>[2x]MAYFDYTSAKPVDERILEAMLPYMTESFGNPSSVHSYGFKAREAVQEAREKVAKLVNGGGGTVVFTSGATEANNLAIIGYAMRNARKGKHILVSAVEHMSVINPAKFLQKQGFEVEYIPVGKYGEVDVSFIDQKLRDDTILVSVQHANNEIGTIQPVEEISEVLAGKAALHIDATASVGQ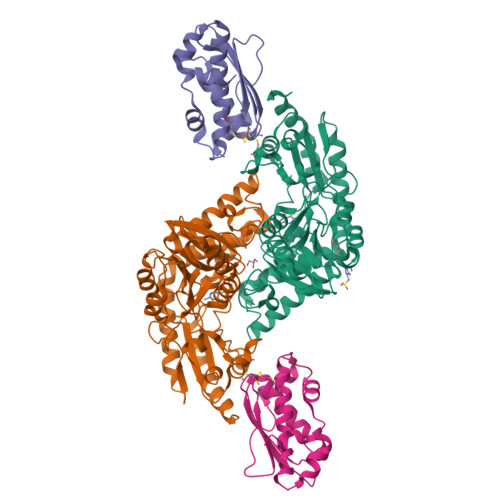IEVDVEKIGADMLTISSNDIYGPKGVGALWIRKEAKLQPVILGGGQENGLRSGSENVPSIVGFGKAAEITAMEWREEAERLRRLRDRIIDNVLKIEESYLNGHPEKRLPNNVNVRFSYIEGESIVLSLDMAGIQASTGSACSSKTLQPSHVLMACGLKHEEAHGTLLLTLGRYNTDEDVDRLLEVLPGVIERLRSMSPLYRR;>[2x]MYSDKVFDHFQNPRNVGKIEDADGVGTVGNPVCGDLMTIYIKVKDNRIEDIKFQTFGCAAAIATSSMATEMAKGKTIEEALKITRDAVAEALGGLPKQKMHCSNLAADALRRAIVDYFRKNGKIDKIKELGLEKELEKMEKGEMDDHGEYCEA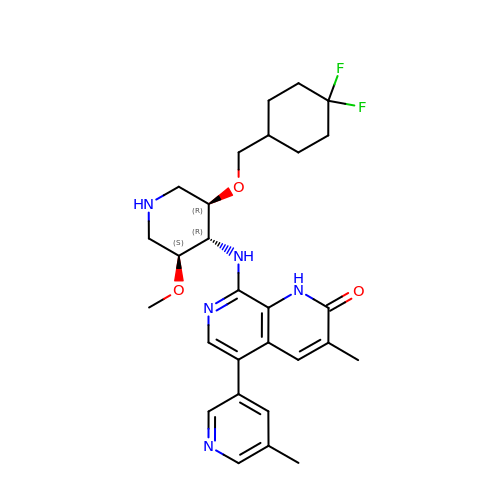8-(((3R,4R,5S)-3-((4,4-difluorocyclohexyl)methoxy)-5-methoxypiperidin-4-yl)amino)-3-methyl-5-(5-methylpyridin-3-yl)-1,7-naphthyridin-2(1H)-one | C28 H35 F2 N5 O3 | YDPMMWAOCCOULO-JBRSBNLGSA-N> MHHHHHHHDGTENPIHDRTSDYHKYLKVKQGDSDLFKLTV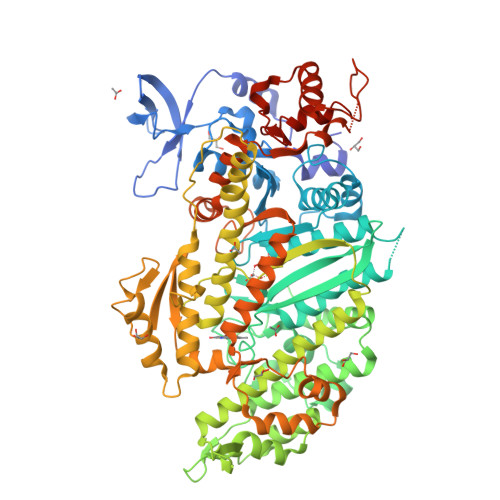SDKRYIWYNPDPKERDSYECGEIVSETSDSFTFKTVDGQDRQVKKDDANQRNPIKFDGVEDMSELSYLNEPAVFHNLRVRYNQDLIYTYSGLFLVAVNPFKRIPIYTQEMVDIFKGRRRNEVAPHIFAISDVAYRSMLDDRQNQSLLITGESGAGKTENTKKVIQYLASVAGRNQANGSGVLEQQILQANPILEAFGNAKTTRNNNSSRFGKFIEIQFNSAGFISGASIQSYLLEKSRVVFQSETERNYHIFYQLLAGATAEEKKALHLAGPESFNYLNQSGCVDIKGVSDSEEFKITRQAMDIVGFSQEEQMSIFKIIAGILHLGNIKFEKGAGEGAVLKDKTALNAASTVFGVNPSVLEKALMEPRILAGRDLVAQHLNVEKSSSSRDALVKALYGRLFLWLVKKINNVLCQERKAYFIGVLDISGFEIFKVNSFEQLCINYTNEKLQQFFNHHMFKLEQEEYLKEKINWTFIDFGLDSQATIDLIDGRQPPGILALLDEQSVFPNATDNTLITKLHSHFSKKNAKYEEPRFSKTEFGVTHYAGQVMYEIQDWLEKNKDPLQQDLELCFKDSSDNVVTKLFNDPNIASRAKKGANFITVAAQYKEQLASLMATLETTNPHFVRCIIPNNKQLPAKLEDKVVLDQLRCNGVLEGIRITRKGFPNRIIYADFVKRYYLLAPNVPRDAEDSQKATDAVLKHLNIDPEQYRFGITKIFFRAGQLARIEEAREQRLESNEPPMDFDDDIPF>[2x]NATEIRASVGKMIDGIGRFYIQMCTELKLSDYEGRLIQNSLTIERMVLSAFDTGGPIYRRVDGKWRRELILYDKEEIRRIWRQANNGDDATAGLTHMMIWHSNLNDATYQRTRALVRTGMDPRMCSLMQGSTLPRR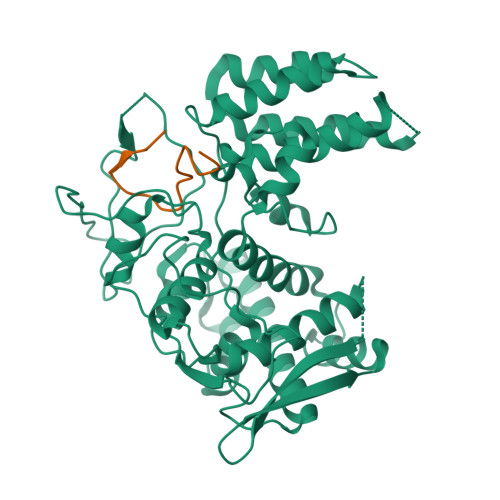SGAAGAAVKGVGTMVMELIRMIKRGINRRTRIAYERMCNILKGKFQTAAQRTMVDQVRESRNPGNAEFEDLIFLARSALILRGSVAHKSCLPACVYGSAVASGYDFEREGYSLVGIDPFRLLQNSQVYSLIRPNENPAHKSQLVWMACHSAAFEDLRVSSFIRGTKVVPRGKLSTRGVQIASNENMETMESSTLELRSRYWAIRTRSGGNTDVSFQGRGVFELSDEKATSPIVPSFDMSNEGSYFF;>SSGQISIQPTFSVQRNLPF[2x]(5~{R})-2-(hydroxymethyl)-3-[(~{E})-non-3-enyl]-5-oxidanyl-cyclohex-2-en-1-one | C16 H26 O3 | 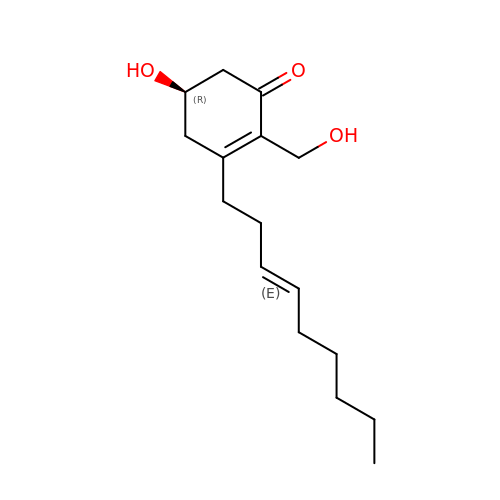UIYPBPASYFNZQB-UHFFFAOYSA-N>DKPVAHVVANHQVEEQLEWLSQRANALLANGMDLKDNQLVVPADGLYLVYSQVLFKGQGCPDYVLLTHTVSRFAISYQEKVNLLSAVKSPCPKDTPEGAELKPWYEPIYLGGVFQLEKGDQLSAEVNLPKYLDFAESGQVYFGVIAL[3x];>VCPQGKY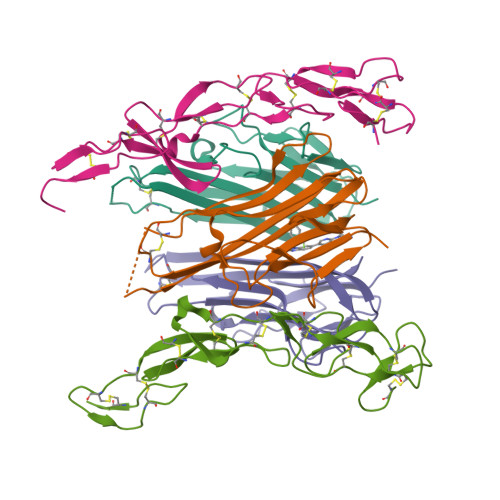IHPQDNSICCTKCHKGTYLYNDCPGPGQDTDCRECESGSFTASENHLRHCLSCSKCRKEMGQVEISSCTVDRDTVCGCRKNQYRHYWSENLFQCFNCSLCLNGTVHLSCQEKQNTVCTCHAGFFLRENECVSSSN[2x]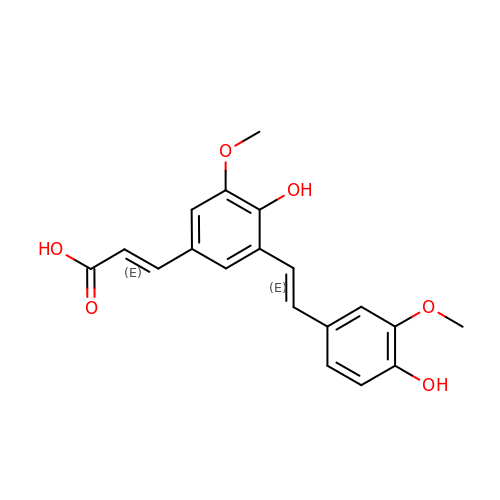(2E)-3-{4-hydroxy-3-[(E)-2-(4-hydroxy-3-methoxyphenyl)ethenyl]-5-methoxyphenyl}prop-2-enoic acid | C19 H18 O6 | SLIMCXCSQXYCGL-JENUQAQBSA-N> MWLFEESAVGFCSNSGVIDNKHAGYTGTGFIDTENAVGASIVWSLSAASAKTYTAQIRFGNGGTSARRATVVVNDSQIKTLDFPTNSNWTQWQTVNVDIPLKAGTNSIKLVAETADGL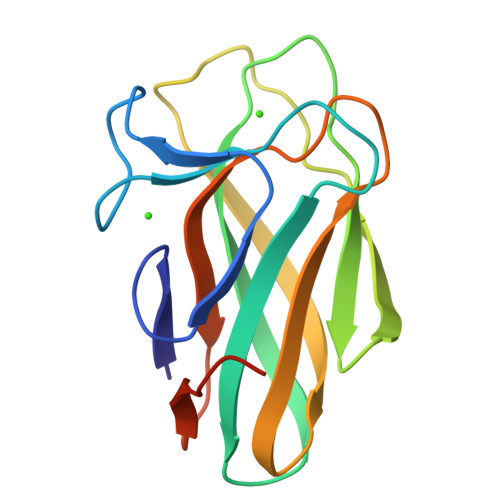ANIDSIRVTGNGITPAACPLEHHHHHH>[4x]SNAMQVKTQSCVVAGKKTVAVTEQTIDWNNNGTLVQITRGGICGSDLHYYQEGKVGNFMIKAPMVLGHEVIGKVIHSDSSELHEGQTVAINPSKPCGHCKYCIEHNENQCTDMRFFGSAMYFPHVDGGFTRYKMVETSQCVPYPAKADEKVMAFAEPLAVAIHAAHQAGELQGKRVFISGVGPIGCLIVSAVKTLGAAEIVCADVSPRSLSL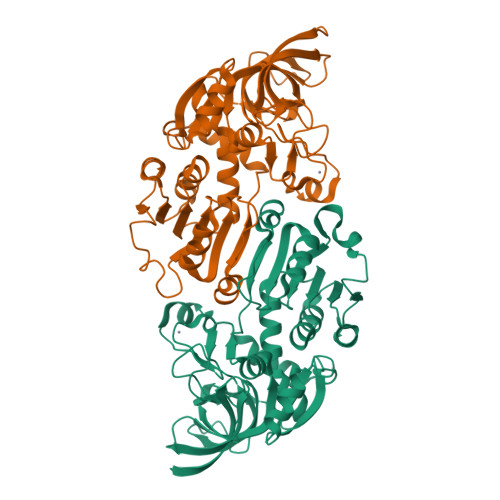GKEMGADVLVNPQNDDMDHWKAEKGYFDVSFEVSGHPSSVNTCLEVTRARGVMVQVGMGGAMAEFPMMTLIGKEISLRGSFRFTSEFNTAVSWLANGVINPLPLLSAEYPFTDLEEALRFAGDKTQAAKVQLVF>[2x]MSQRITIDPVTRIQGHLRIDCEIENGVVSKAWASGTMWRGMEEIVKNRDPRDAWMIVQRICGVCTTTHALSSVRAAESALNIDVPVNAQYIRNIILAAHTTHDHIVHFYQLSALDWVDITSALQADPTKASEMLKGVSTWHLNSPEEFTKVQNKIKDLVASGQLGIFANGYWGHPAMKLPPEVNLIAVAHYLQALECQRDANRVVALLGGKTPHIQNLAVGGVANPINLDGLGVLNLERLMYIKSFIDKLSDFVEQVYKVDTAVIAAFYPEWLTRGKGAVNYLSVPEFPTDSKNGSFLFPGGYIENADLSSYRPITSHSDEYLIKGIQESAKHSWYKDEAPQAPWEGTTIPAYDGWSDD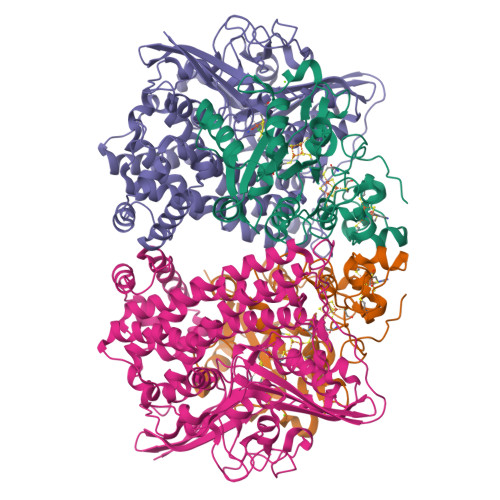GKYSWVKSPTFYGKTVEVGPLANMLVKLAAGRESTQNKLNEIVAIYQKLTGNTLEVAQLHSTLGRIIGRTVHCCELQDILQNQYSALITNIGKGDHTTFVKPNIPATGEFKGVGFLEAPRGMLSHWMVIKDGIISNYQAVVPSTWNSGPRNFNDDVGPYEQSLVGTPVADPNKPLEVVRTIHSFDPCMACAVHVVDADGNEVVSVKVL;>[2x]EMAESVTNPQRPPVIWIGAQECTGCTESLLRATHPTVENLVLETISLEYHEVLSAAFGHQVEENKHNALEKYKGQYVLVVDGSIPLKDNGIYCMVAGEPIVDHIRKAAEGAAAIIAIGSCSAWGGVAAAGVNPTGAVSLQEVLPGKTVINIPGCPPNPHNFLATVAHIITYGKPPKLDDKNRPTFAYGRLIHEHCERRPHFDAGRFAKEFGDEGHREGWCLYHLGCKGPETYGNCSTLQFCDVGGVWPVAIGHPCYGCNEEGIGFHKGIHQLANVENQTPRSQKPDVNAKEGGRSHHHHHH> SHMSKAKFDKAVEIVQSLPKDGPIKPTQDEQLYFYKYFKQATVGDVNISRPGLMDFTGKAKWDAWKSVEGTSKEVAYQK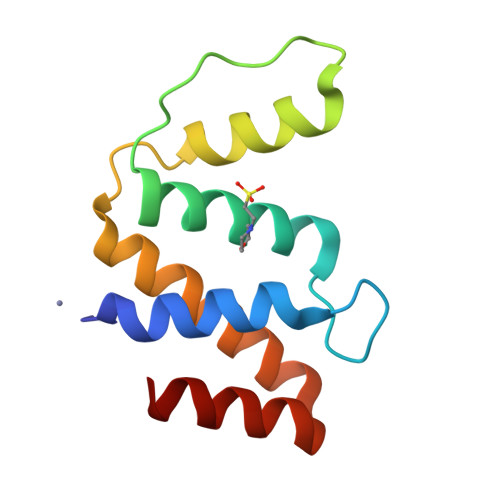YVEKLLEILKKADTEESKKYIAEIEAA>[4x]GSSHHHHHHSSGLVPGGSHMVSKGEENNMAVIKPDMKIKLRMEGAVNGHPFAIEGVGLGKPFEGKQSMDLKVKEGGPLPFAYDILTTVFCYGNRVFAKYPEN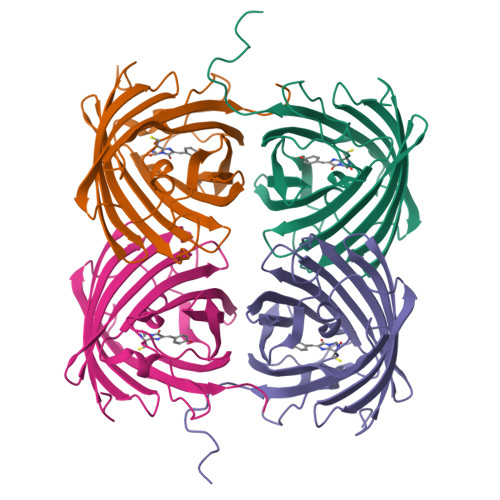IVDYFKQSFPEGYSWERSMNYEDGGICNATNDITLDGDCYIYEIRFDGVNFPANGPVMQKRTVKWEPSTEKLYVRDGVLKGDVNTALSLEGGGHYRCDFKTTYKAKKVVQLPDYHFVDHHIEIKSHDKDYSNVNLHEHAEAHSGLPRQAMDELYK>GPGSMSNVAVNTVFASLDNFRKGTVEIISGEARHYAFSNIFEVAQNSKPYEKVVVGLNLGYVVE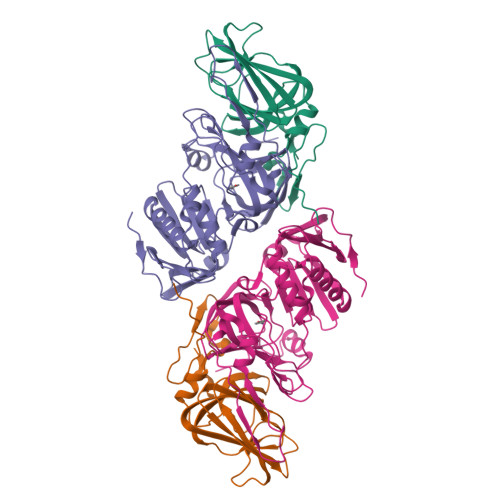TLRAEGQSPWFTAAHDEFAIVMDGEVRVEFLKLDAPSKHGEGTHLAGELPVGKPMGYVLLKRGHQCLLPAGSAYRFEASRPGVILQQTIKGPLSVEKWAEICLK[4x];>MAMLESAVDSAAFADDDVQASPPHAVTGYRSFQLGAFELSRDEYFARITWPAKGETRSHLIPADIFLRAMMRDVAWGFFYGWVNFDHVIGTRNYYGKVDLYAGTFNGTLKAAGVNYTENFETPLIMATFKAILRDWTNATFDPFAAPEETGSAFGRKNGENLECIERFRIATKRMPGLQDDSPLRNDLPVNRQFADVSQDEPEVHAAEGFEGELHAFSLFKYLSRSDVTWNPSVTSVCKASLFCPTTEEFILPVFHGNDRVEWFIQMSDEIVWDVGDKDDGNPRARITMRAGDVCAMPADIRHQGYSTKRSMLMVWENATPNLPHLYESGELKPYPIEF[4x]>[2x]MIKDKCFEGVRFEQQDLEGEQFQGCRFIGCNFSWLDLAECRFVDCSF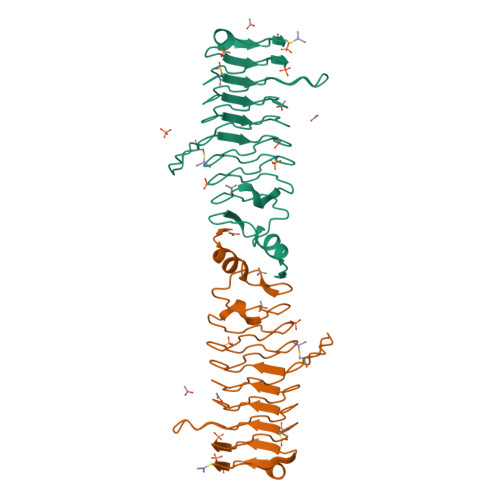YDRESEQSCLLQGCDLREASFLRCDLTMADCSRSQCLGLELRDCQALGINFSRASFANQITVKSYFCEAHLTGNNFSYANFEGCLLEQCELSGNRWQGANLFGASLAGSDLSGSEFGQIDWASVNLQGCDLRQCDLPGLDLRRVNLDGVQINEDQQQALLEQIGLIVFP>[4x]MMTRKKELAIALS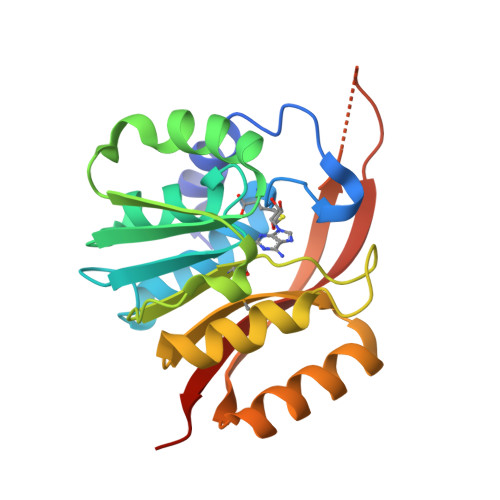KLKGFKNPKVWLEQYRTPGNAASELLWLAYSLGDIEGKVVADLGAGTGVLSYGALLLGAKEVICVEVDKEAVDVLIENLGEFKGKFKVFIGDVSEFNSRVDIVIMNPPFGSQRKHADRPFLLKAFEISDVVYSIHLAKPEVRRFIEKFSWEHGFVVTHRLTTKIEIPLQFFFHRKKLERITVDIYRFSKVINSR>GAMSHPHDSKVFPDLPEHQDNPSQLRLQHDGLATDDKARLEPMCLAEYLISGPGGMDPDIEIDDDTYDECREVLSRILEDAYTQSGTFRRLMNYAYDQELHDVEQRWLLGAGENFGTTVTDEDLESSEGRKVIALNLDDTDDDSIPEYYESNDGPQQFDTTRSFIHQVVHALTHLQDKEDSNPRGPVVEYTNIILKEMGHTSPPRIAYEFSN[2x]

Here, we report that the zinc metalloprotease T3SS effector proteins GtgA, GogA, and PipA from S. enterica cleave a subset of NF-κB subunits comprising p65, RelB, and cRel, whereas NleC from EPEC/EHEC cleaves all five NF-κB subunits. GtgA, in both its apo-form and in complex with p65, has a globular structure, with the catalytic core assuming a Zincin-like fold. The active-site helix (αG) sits at the bottom of a cleft formed between an upper NSD and a lower CSD. Similar to NleC, the active-site cleft of GtgA is highly negatively charged, and the active-site cleft mimics the shape of the DNA major groove.

The structure of Zn2+-bound GtgA(20–228)E183Q was solved at 2.6 Å resolution by molecular replacement using the coordinates of GtgA in complex with p65. No electron density was visible for residues 20–24, 157, and 158 and the C-terminal Asn-228. GtgA(20–228)E183Q crystals belong to space group I121 with two molecules in the a.u. that overlap with a root mean square deviation (RMSD; Cα of residues 27–154 and 160–227) of 0.2 Å. The two molecules are covalently linked by a disulfide bond between Cys-44 of each chain. This is likely a crystallization artifact, as the elution volume of GtgA(20–228)E183Q following size-exclusion chromatography was indicative of a monomeric protein, and the disulfide bond is absent in the structure of the GtgA–p65 complex. In the GtgA apo structure, Tyr-224 is 3.9 Å from the active-site zinc, suggesting that this residue, which is conserved in GogA, PipA, and NleC, stabilizes the tetrahedral intermediate. The active site of GtgA is surrounded by a large negatively charged surface formed by αF, the upper rim residues, and the loop connecting helices αC and αD, which folds down over the incomplete ψ-loop. An overlap of the apo-GtgA with the GtgA chain in the complex structures demonstrates that this region clashes sterically with residues in the p65 NTD chain. In GtgA, the ψ-loop motif is incomplete as, in both the complex and apo structures, the lowermost strand residues Phe-131 to Val-135, which form the upper rim, are not in the β-sheet.VhCBP is a periplasmic chitooligosaccharide-binding protein mainly responsible for translocation of the chitooligosaccharide (GlcNAc)2 across the double membranes of marine bacteria. The chitooligosaccharide-specific SBP is localized to the periplasmic compartment of the bacterial cell wall and serves as a mobile component of the (GlcNAc)2-specific ABC transporter. SBPs share a common structural feature comprising two domains connected by a flexible hinge region. VcCBP and VhCBP belong to cluster C/subcluster IV (C-IV), members of which are specific for oligosaccharides, including mannooligosaccharides, cellooligosaccharides, and chitooligosaccharides.

A remarkable structure was seen with W513A, in which the substrate-binding groove was partially open at the reducing-end side (site 2). The domain movement of W513A released bound water molecules trapped by several hydrogen bonds with the main-chain carbonyl of His7, the main-chain -NH of Ser220, the side chain Oγ of Ser221, and the N-acetyl carbonyl group of the nonreducing end GlcNAc, while the water molecules were retained in the other mutant structures. Trp513 is located at the mouth of the GlcNAc-binding groove, and its position is thought to regulate the translocation of (GlcNAc)2 to the (GlcNAc)2-specific ABC transporter. In fact, the crystal structure of the W513A mutant showed a ‘half-open’ conformation, which effectively provides a snapshot of the sugar-releasing process that facilitates translocation. The W363A mutation had a large effect on the enthalpic term, while in W513A, a large change was observed in the entropic contribution. Trp363 interacts purely through CH-π stacking, while Trp513 interacts through both CH-π stacking and hydrogen bonding with the N-acetyl group of the GlcNAc in site 1. The crystal structure of the W513A–(GlcNAc)2 complex observed in the present report is the first experimental evidence capturing an intermediary conformation between fully closed and fully open conformations in the sugar translocation pathway. Our ITC data suggested the closed (sugar-bound) state has high affinity to the (GlcNAc)2 substrate (Kd of 0.03 μM), while the semiopen state has 1200 lower affinity than the closed state (Kd of ~37 μM). We propose that this decrease in the binding affinity facilitates the sugar release from the VhCBP to its membrane-transporting partner. The structure of the W513A–(GlcNAc)2 complex in a ‘half-open’ conformation unveiled the intermediary step of the (GlcNAc)2 translocation from the soluble CBP in the periplasm to the inner membrane–transporting components.

> AERSELTIHPKEFTTFVRNFNPFLGATNLHTTTDFIYEPLVVFNEMHGNTPVFRLAENFQMSDDLMSVTFDIRKGVKWSDGEAFTADDVVYSFNLVKEKPELDQSGINSWVTGVEKVNDYQVKFRLSEANSNVPYEIAKVPVVPKHVWSKVKDPSTFTNENPVGSGPFTVIDTFTPQLYIQCENPNYWDAANLDVDCLRVPQIANNDQFLGKVVNGEMDWTSSFVPDIDRTYAAASPKHHYWYPPAGTQAFVVNFKNPDAAKNEALTNVDFRRAFSMALDRQTIIDIAFYGGGTVNDFASGLGYAFEAWSDEKTHDKFKAYNSYNAEGAKKLLAKAGFKDVNKDGFVDTPSGKSFELLIQSPNGWTDFNNTVQLAVEQLAEVGIKARARTPDFSVYNQAMLEGTYDVAYTNYFHGADPYTYWNSAYNSALQSGDGMPRFAMHFYKNEKLDGLLNSFYKTADKQEQLEIAHGIQQIIAQDQVTIPVLSGAYMYQYNTTRFTGWWNEENPKGRPNIAAGIPERLLHVLDLKPVKHHHHHH> HKCDITLQEIIKTLNSLTEQKTLCTELTVTDIFAASKNTTEKETFCRAATVLRQFYSHHEKDTRCLGATAQQFHRHKQLIRFLKRLDRNLWGLAGLNSCPVKEANQS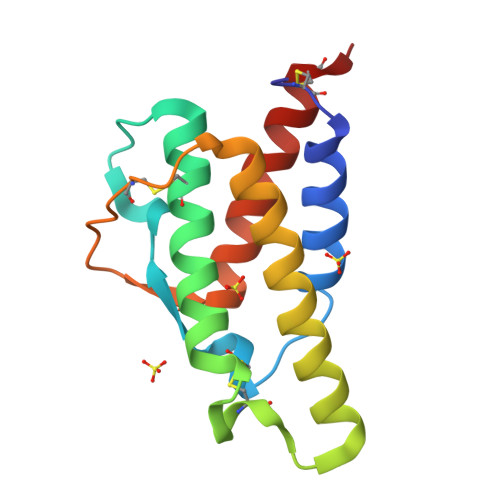TLENFLERLKTIMREKYSKCSS>MTLEQAIERAGTKHGNKGWEAALSAIEMANLFKSLRGTGGSGSSMEIYEGKLTAEGLRFGIVASRFNHALVDRLVEGAIDCIVRHGGREEDITLVRVPGSWEIPVAAGELARKEDIDAVIAIGVLIRGATPHFDYIASEVSKGLANLSLELRKPITFGVITAD[150x]

As such, we found that a circularly permuted variant of a cage-forming enzyme, Aquifex aeolicus lumazine synthase, cpAaLS, assembles into a variety of hollow spherical and cylindrical structures in response to changes in ionic strength. Cryogenic electron microscopy revealed that these structures are composed entirely of pentameric subunits, and the dramatic cage-to-tube transformation is attributed to the moderately hindered 3-fold symmetry interaction and the imparted torsion angle of the building blocks, where both mechanisms are mediated by an α-helix domain that is untethered from the native position by circular permutation. While the wild-type protein, AaLS-wt, self-assembles into a ∼ 16 nm dodecahedral structure composed of 60 identical monomers,35 the negatively supercharged variants AaLS-neg and AaLS-13 adopt expanded 360- and 720-mer assemblies, respectively, constructed entirely from pentameric capsomers. Moreover, a circularly permuted variant of AaLS, cpAaLS(119), forms not only ∼24 nm and ∼28 nm expanded spherical cages, but also straight ∼24 nm-wide tubes of variable length. We previously designed two circularly permuted variants of AaLS and confirmed that their morphologies depend on the positions of the newly generated N- and C-termini. The native terminal amino acids were connected via an octapeptide linker using genetic fusion and new sequence termini were introduced either between residues 84 and 85 or 119 and 120, yielding cpAaLS(84) or cpAaLS(119), respectively.

While remaining as unassembled fragments in the absence of salt, adding 0.15 M NaCl facilitated cpAaLS(119) tubular formation with ∼92% yield. In the tubular structure, the pentameric building blocks are arranged as a triple-stranded helix, which is unique and has never been seen for any natural or engineered proteins. While the number of pentamer–pentamer contacts remains 0 or 1 without NaCl at pH 8.5, judged by the 2D-averaged cryo-EM images, the mean contact number per pentamer increases to 3, 3.7, and 4 in the tubular, 28 nm-, and 24 nm spherical cages, respectively. In the cpAaLS(119) tubes, the “untethered” α-helix(120–131) binds to the adjacent pentamer surface, which is a solvent-exposed region in wild-type-like assemblies. Because of this non-native interaction, the α-helix(120–131) appears to block 3-fold symmetrical pentamer–pentamer interactions, which explains the uncontacted interfaces observed in the cpAaLS(119) assemblies. Furthermore, substantial cryo-EM density corresponding to the α-helix(120–131) was found only for 2 protomers in each pentamer constituting the tubular assembly, and invisible in the spherical assemblies. In both the straight and twisted tubes, the pentamer–pentamer interaction adopts a wide range of torsion angles: −35°, 18°, and 24° for the straight tube, for example.>GHHHHHHHHHHSSGHIEGRHMRVLFASLGTHGHTYPLLPLATAARAAGHEVTFATGEGFAGTLRKLGFEPVATGMPVFDGFLAALRIRFDTDSPEGLTPEQLSELPQIVFGRVIPQRVFDELQPVIERLRPDLVVQEISNYGAGLAALKAGIPTICHGVGRDTPDDLTRSIEEEVRGLAQRLGLDLPPGRIDGFGNPFIDIFPPSLQEPEFRARPRRHELRPVPFAEQGDLPAWLSSRDTARPLVYLTLGTSSGGTVEVLRAAIDGLAGLDADVLVASGPSLDVSGLGEVPANVRLESWVPQAALLPHVDLVVHHGGSGTTLGALGAGVPQLSFPWAGDSFANAQAVAQAGAGDHLLPDNISPDSVSGAAKRLLAE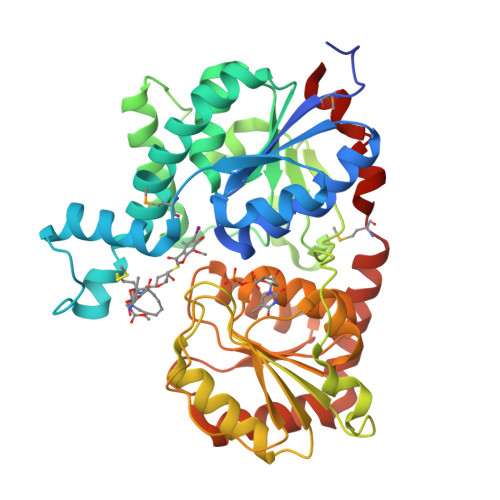ESYRAGARAVAAEIAAMPGPDEVVRLLPGFASRSAG[2x]> SSIMKILLIGDVGVGKSCLLVRFVEDKFNPSFITTIGIDFKIKTVDINGKKVKLQLWDTAGQE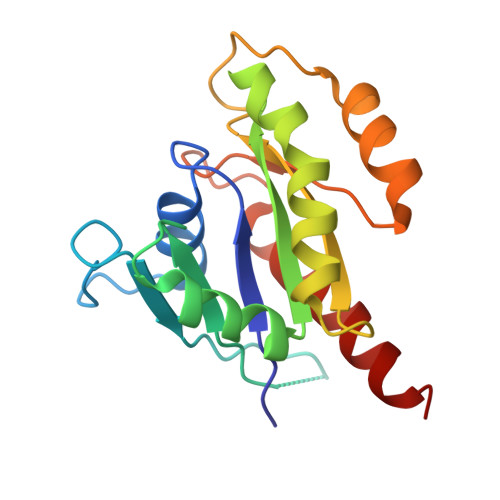RFRTITTAYYRGAMGIILVYDVTDERTFTNIKQWFKTVNEHANDEAQLLLVGNKSDMETRVVTADQGEALAKELGIPFIESSAKNDDNVNEIFFTLAKLIQEKIDSN>[2x]MGNLTGNSKKAADSGDKPVIKMYQIGDKPDNLDELLANANKIIEEKVGAKLDIQYLGWGDYGKKMSVITSSGENYDIAFADNYIVNAQKGAYADLTELYKKEGKDLYKALDPAYIKGNTVNGKIYAVPVAANVASSQN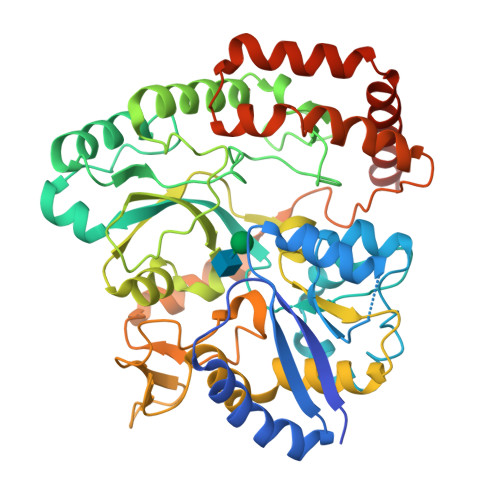FAFNGTLLAKYGIDISGVTSYETLEPVLKQIKEKAPDVVPFAIGKVFIPSDNFDYPVANGLPFVIDLEGDTTKVVNRYEVPRFKEHLKTLHKFYEAGYIPKDVATSDTSFDLQQDTWFVREETVGPADYGNSLLSRVANKDIQIKPITNFIKKNQTTQVANFVISNNSKNKEKSMEILNLLNTNPELLNGLVYGPEGKNWEKIEGKENRVRVLDGYKGNTHMGGWNTGNNWILYINENVTDQQIENSKKELAEAKESPALGFIFNTDNVKSEISAIANTMQQFDTAINTGTVDPDKAIPELMEKLKSEGAYEKVLNEMQKQYDEFLKNKKLEHHHHHH> G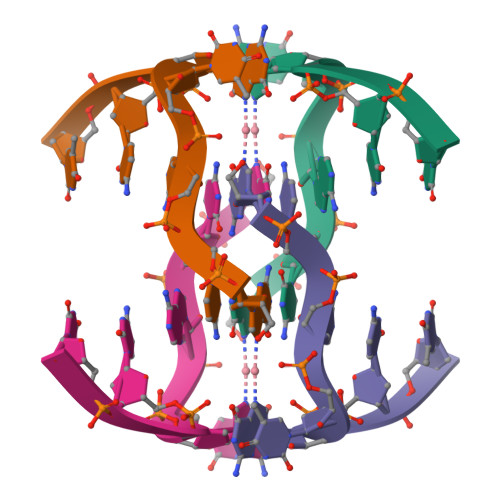CATGCT> TTMDVQSAADDTGLPMLVVRGPFNVVWQRLPAALEKVGMKVT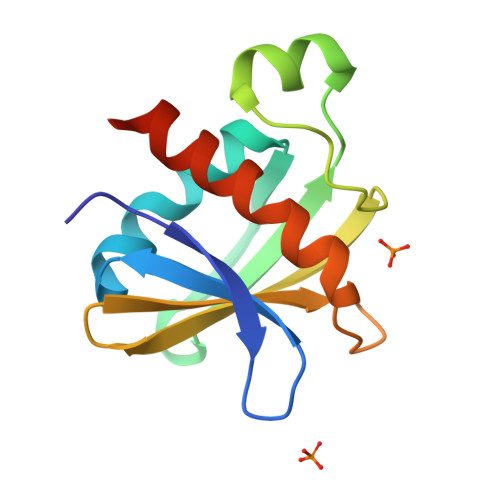DSTRSQGNMAVTYKPLSDSDWQELGASDPGLASGDYKLQVGDLDNRSSLQFIDPKGHTLTQSQNDALVAVFQAAFSKLEHHHHHH> GPGSNTMARAKILQD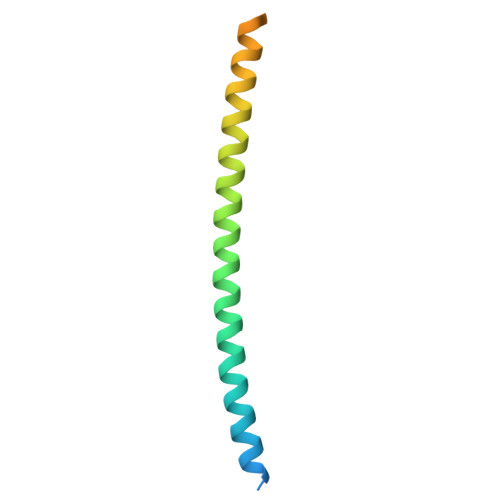IDRELDLVERESAKLRKKQAELDEEEKEIDAKLRYLEMGINRRKEALLKEREKRERAYLQGVAEDRDYMSDSEVSS>[6x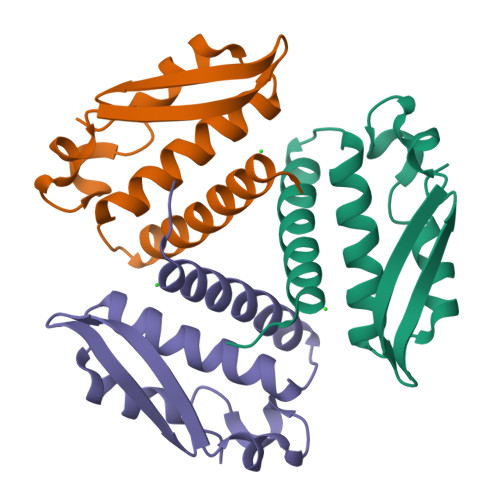]GPGSMHLTPREFDKLVIHMLSDVALKRKNKGLKLNHPEAVAVLSAYVLDGAREGKTVEEVMDGARSVLKADDVMDGVPDLLPLIQVEAVFSDGSRLVSLHNPIT>[3x]VINTLDGV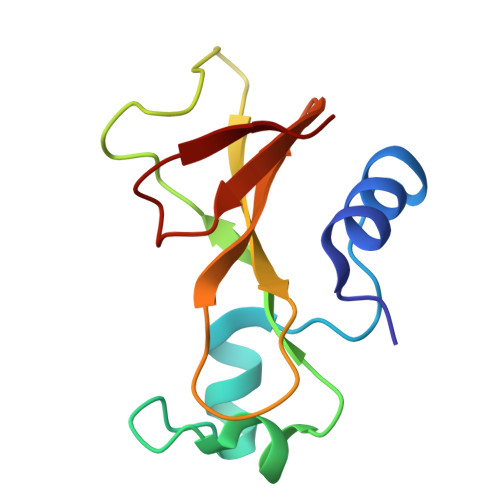ADYLQTYHKLPDNYITKSEAQALGWVASKGNLADVAPGKSIGGDIFSNREGKLPGKSGRTWREADINYTSGFRNSDRILYSSDWLIYKTTDHYQTFTKIR>SNAMIDGKFISAIITAAGSGLRMRSKINKPYIEVGGRKVLEITLDTVSRVKEIDEIILVIRKDDEDIIKDILEKYDGNIRYVYGSTTRELSTFEGLKALDPQSELVLTHDGVRPFASEELFLKTINALRKNKAVITATKSKDTVKIIDDDMYVDFTPNRDYVYNIQTPQAFDKKLIYAM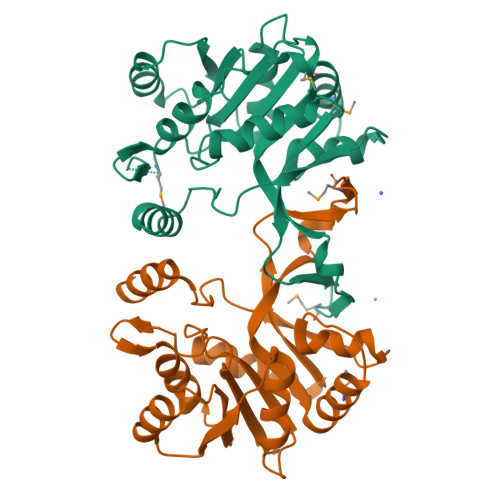YEKYLASEFKVTDDSQLFEFFDRDEKVKVVHGEYSNIKITTQEDIIFANAYLQRKKDV[2x]(2R,3R,4S,5R)-5-({[(R)-{[(R)-{[(2R,3S,4R,5R)-5-(6-AMINO-9H-PURIN-9-YL)-3,4-DIHYDROXYTETRAHYDROFURAN-2-YL]METHOXY}(HYDROXY)PHOSPHORYL]OXY}(HYDROXY)PHOSPHORYL]OXY}METHYL)-3,4-DIHYDROXYTETRAHYDROFURAN-2-YL ACETATE | C17 H25 N5 O15 P2 | 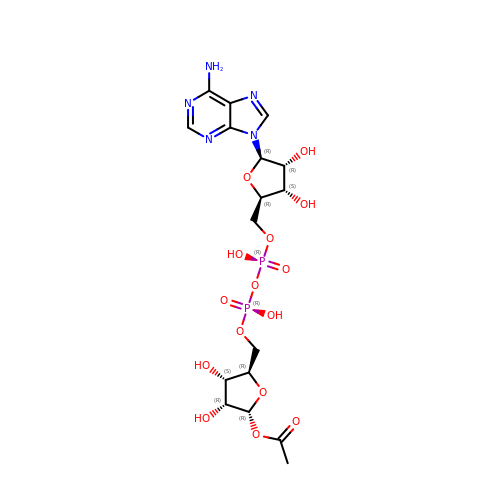IJOUKWCBVUMMCR-DLFWLGJNSA-N6-ETHYL-5-PHENYLPYRIMIDINE-2,4-DIAMINE | C12 H14 N4 | 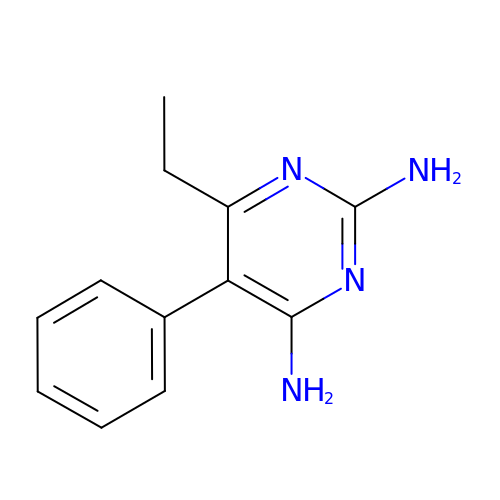XREDUPOVEQDQQS-UHFFFAOYSA-N5'-O-{3-[3-(2-carboxyphenyl)-3-oxopropyl]phenyl}adenosine 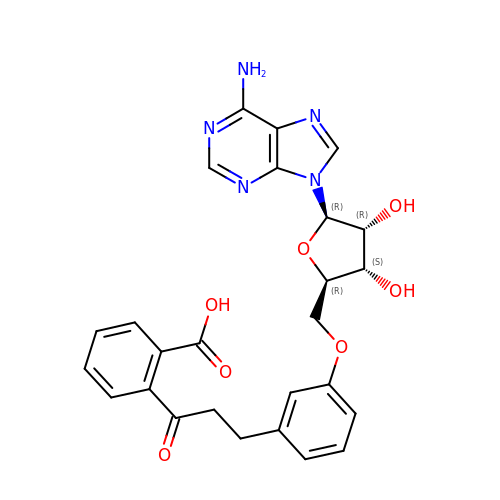| C26 H25 N5 O7 | GEMGRSMVWNUQGG-PTGPVQHPSA-N>[6x]SAAQKFVKQVIREAFLQDASDIHIEPRQNDVQVRLRIDGALRPYSTLPKGALNAVISVVKIMGGLNIAEKRLPQDGRVRYREGAIDVDLR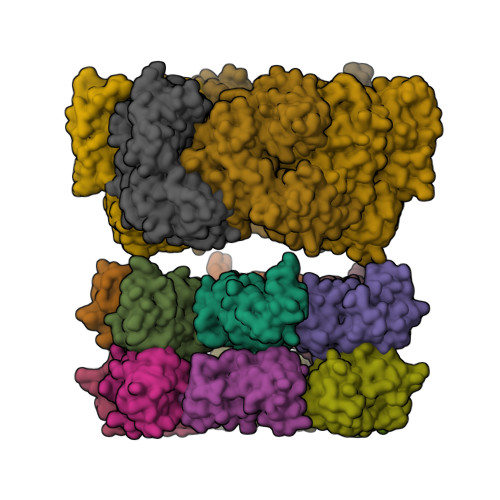LSTLPTVYGEKAVMRLLKKASDIPEIEDLGFAPGVFERFKEVISKPYGIFLITGPTGSGKSFTTFSILKRIATPDKNTQTIEDPVEYEIPGINQTQVNPQAGLTFARALRAFLRQDPDIIMVGEIRDSETAKIATEAALTGHLVIATLHTNDAAQAITRLDEMGVEPFNISAALIGVLSQRLVRRVCEHCKVEVKPDPETLRRLGLSEAEIQGARLYKGMGCERCGGTGYKGRYAIHELLVVDDEIRHAIVAGKSATEIKEIARRKGMKTLREDGLYKALQGITTLEEVLARTIEAAAELALVPRGSSAHHHHHHHHHH;>[6x]LPRAKPLGEILVELGLARPEDVEEALQKQRRGGGRLEDTLVQSGKLRPEALAQAVATQLGYPYVDPEEDPPDPGAPLLLPEDLCRRYGVFPHRLEGNRLVLLMKDPRNILALDDVRLALKRKGLNYEVAPAVATEAAITKLIERFY;>QKDLKLGELLLQKGWISREALEEALVEQEKTGDLLGRILVRKGLPEEALYRALAEQKGLEFLESTEGIVPDPSAALLLLRSDALRYGAVPIGFQNGEVEVVLSDPRHKEAVAQLLNRPARFYLALPQAWEELFRRAY[6x]> GSPEFMAQILPIRFQEHLQLQNLGINPANIGFSTLTMESDKFICIREKVGEQAQVVIIDMNDPSNPIRRPISADSAIMNPASKVIALKAGKTLQIFNIEMKSKMKAHTMTDDVTFWKWISLNTVALVTDNAVYHWSMEGESQPVKMFDRHSSLAGCQIINYRTDAKQKWLLLTGISAQQNRVVGAMQLYSVDRKVSQPIEGHAASFAQFKMEGNAEESTLFCFAVRGQAGGKLHIIEVGTPPTGNQPFPKKAVDVFFPPEAQNDFPVAMQISEKHDVVFLITKYG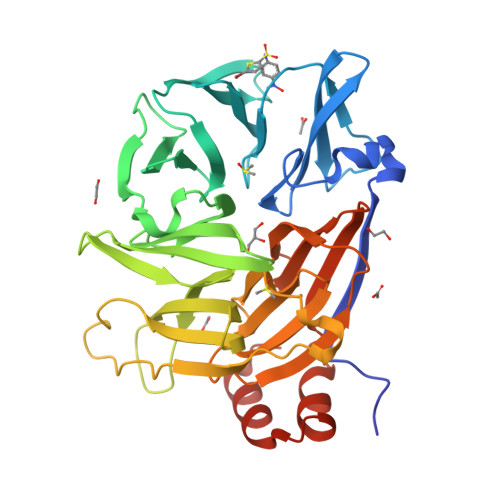YIHLYDLETGTCIYMNRISGETIFVTAPHEATAGIIGVNRKGQVLSVCVEEENIIPYITNVLQNPDLALRMAVRNNLAGAEELF> 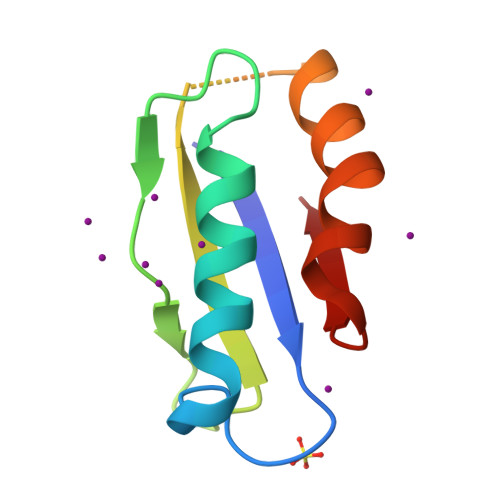PVQVLVRFDAGGASAPEHSQTIAAIRHRIAQAPNVVSVAPPRFADDNGSALLSAVLSVDPEDLGARDTITWMRTQLPRVAGAAQVDVG>[3x]SNAMKLGALISESRNPDTMDLDTLSTLEMLTRINDEDRKVPEAIRLVIPNIAQAVDLAAKALRDGGRLIYLGAGTSGRLGVLDASECPPTFGVPHGRVIGLIAGGPGALLKAVEGAEDDVSLGERDLRDLQLTATDMVVGLAASGRTPYVIGALRFARQLGCPTAAISCNPDSPIAQEALVAISPVVGPEALTGSTRM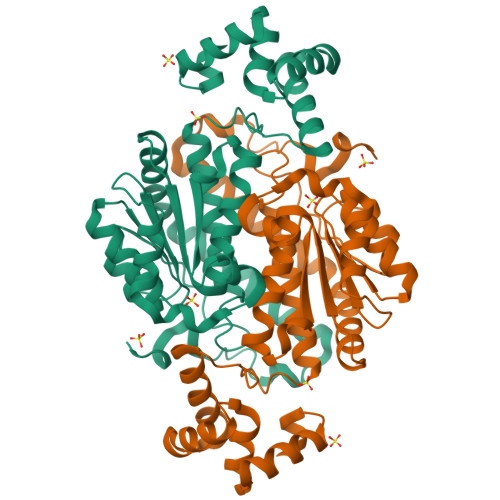KSGTAQKLVLNMLSTGAMVKLGKVYQNLMVDVKATNVKLVDRACRIVVEATGASRVEAENALSQTEFEVKPAILMILKGVSVEQARLNLQQHNGYLRAAL>[12x]MSEY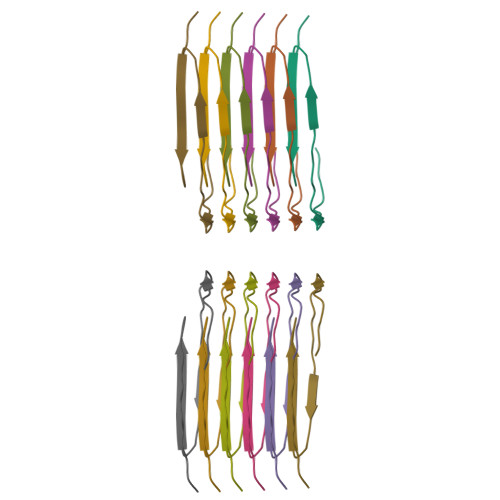IRVTEDENDEPIEIPSEDDGTVLLSTVTAQFPGACGLRYRNPVSQCMRGVRLVEGILHAPDAGWGNLVYVVNYPKDNKRKMDETDASSAVKVKRAVQKTSDLIVLGLPWKTTEQDLKEYFSTFGEVLMVQVKKDLKTGHSKGFGFVRFTEYETQVKVMSQRHMIDGRWCDCKLPNSKQSQDEPLRSRKVFVGRCTEDMTEDELREFFSQYGDVMDVFIPKPFRAFAFVTFADDQIAQSLCGEDLIIKGISVHISNAEPKHNSNRQLERSGRFGGNPGGFGNQGGFGNSRGGGAGLGNNQGSNMGGGMNFGAFSINPAMMAAAQAALQSSWGMMGMLASQQNQSGPSGNNQNQGNMQREPNQAFGSGNNSYSGSNSGAAIGWGSASNAGSGSGFNGGFGSSMDSKSSGWGM A major biofilm matrix determinant of Pseudomonas aeruginosa is the partially deacetylated α-1,4 linked N-acetylgalactosamine polymer, Pel. Once in the periplasm, the large 948-residue protein PelA modifies Pel using its two enzymatic domains. PelA's deacetylase domain selectively removes acetyl groups from the polysaccharide, rendering Pel cationic, while its glycoside hydrolase (GH) family 166 (GH166) domain hydrolyzes Pel. The hydrolase activity is required for the generation of the cell-free form of the polysaccharide, which is important for the biomechanical properties of the biofilm and P. aeruginosa virulence.

Herein, we present the crystal structure of PelA from Pseudomonas thermotolerans (PtPelA) and show that the protein has a unique four-domain structure. Diffraction data were collected for selenomethionyl-incorporated (SeMet) PtPelA at the National Synchrotron Light Source-II to 2.1 Å, and the structure was solved using the single-wavelength anomalous diffraction method. Structural analysis of PtPelA reveals four distinct domains that align well with the AF2 model of PaPelA (PaPelAAF2; 1.6 Å RMSD over 816 α-carbons). Upon analysis of the PtPelA structure, we found that residues 293 to 498 form a mixed α/β domain with 12 β-strands. In our crystal structure, we were unable to model residues 588 to 614 and 703 to 719. Modeling of these residues by AF2 in PaPelAAF2 suggests that these unstructured loops are important for forming a 23 Å-deep, 44 Å-long binding groove. PtPelA also contains a 14-stranded β-rich region comprised of two distinct regions (residues 793–937). Combined, this suggests that the β-rich domain could provide structural stability to PtPelA and facilitate carbohydrate binding. When submitting the structure of PtPelA to the DALI server, only structures of the isolated hydrolase or deacetylase domains of enzymes were identified. These results suggest that the domain organization in the full-length structure of PtPelA is unique with respect to experimentally solved structures. Using sequence analysis and enzymatic assays, we found that PtPelA and its homologs define a new class of carbohydrate esterases, CE21, with distant homology to the CE4 and CE18 families.

> KPSSVAFWYAEQPPLAELSQFDWVVLEPGHADAADIAYLKAQGSTPFAYLSVGEFDGDTAELAGAGLEEGASAVRNDAWHSQVMDLSSSVWREHLFSRAAELRRQGYAGLFLDTLDSFQLQSEDRHEPQRQALVSLLAELHRREPQLSLFFNRGFEVLPELPGVASAVAVESIHAGWEAASSRYRTVSQEDRDWLQPHLEALRAQGVPLVAIEYLPPERREEARELAARLVKEGFIPYVTTPALDTLGVGSLEVQPRRIALVYDPREGELESNPGHVMLGGLLEYLGYRVDYWPAGEALPQRPLKGLYAGVVIWMTSGPPSASDSFHAWLNARIDEQVPIAFLAGLPVDNDGLLQRLGMRRLSQPLRGEPRLEFHDQSLLGAFEAPLRLRTRDLPALTVTDPQLTQAALVLEHGGRRYVPVATGTWGGIALAPYLVEEALDHRRWIIDPFAFIQRAFALPPLPSPDVTTENGRRVATVHIDGDGFVSRAEVPGTPYAGQQVLEAFIRPYPLLTSVSVVEGEVGPKGMYPHLSKELEPIARRIFADPKVEVASHTFSHPFFWQPEKAAQSDDFDPQYGLMMKIPGYEVLDMRREVVGTRDYINQRLTTPEKPVKMIFWSGDALPDAETIKLAYDSGLPNVNGGNTMLTKAYPSLTGLYPLIRPTSGGVQYYAPIINENVYTNLWTGPYYGFRDVLDTFALTDQPRRLRGLHLYYHFYSGTKQASIRAMHQIYAEMLRQQPLSLWMSDYVRRLEGLHCASLARRADGRWQLRGLAGLRTLRLDPALGWPDLARSKGVAGVRDLPQGRYVHLSRADALLALRSSRDPRPALEEANLPLTAWEYRSASQVSFSFAGELPLQFSVRAAGPCRVTVAGQSFQGKEHDGLWRFQLPMKQVRDGQLVC We recently characterized a novel roseophage, vB_DshS-R4C (R4C), that could infect the Dinoroseobacter shibae DFL12T, a ubiquitous group of Gram-negative α-proteobacteria of the Roseobacter clade. Here, we report the atomic capsid and in-situ structures of the tail machine of the marine siphophage, vB_DshS-R4C (R4C), which infects Roseobacter. The R4C virion, comprising 12 distinct structural protein components, has a unique five-fold vertex of the icosahedral capsid that allows genome delivery. In this study, we use cryo-electron microscopy (cryo-EM) and structure prediction to determine the atomic structure of the phage R4C capsid and the in-situ structure of the tail machinery to characterize the distinguished long rigid tail.

The C12 reconstruction of the portal-adaptor complex, with an overall resolution of 4.7 Å, characterizes an adaptor architecture that decorates an accessory Ig-like domain at its periphery. The R4C portal protein, forming a canonical cone-shaped dodecamer with a height of 10 nm, shows considerable structural similarity with portal proteins of other phages, despite poor sequence conservation. The portal protein, characterized from top to bottom, comprises separate crown (residues 476–551), wing, stem, and clip domains (324–376)51. A typical tunnel loop connecting α8 forms the narrowest channel with a diameter of ~30 Å; an analogous structural feature (e.g., phages SPP1 and T4) confines the DNA and prevents its reflux from the capsid, with the specific conformational rearrangement in the tunnel loop regulating genome release. The clip domain, straddling the thick capsid wall, is partially exposed outside the R4C head and interacts with the adaptor proteins. The portal complex is capped by a dodecameric adaptor, which is located outside the capsid shell and interacts with both the portal and the capsid MCPs. Following the nomenclature established for the RcGTA adaptor, the R4C adaptor protein can be divided as: attachment domain (1–106), tube domain, adaptor loop (131–148) and C-terminal hook (167–178). The N-terminus of the adaptor protein is an immunoglobulin (Ig)-like domain (attachment domain), and this domain is connected to the tube domain by a long, flexible loop. The tube domain consists of two α-helices, with the α2 sandwiched between loops from adjacent portal proteins. The tube domain extends the C-terminal hook to the portal clip domain, forming an interaction network comprising five hybrid β-sheets.

>[12x]MRFWPFSKTTNAATRAEPMVTRPDTAPRVRSYRAAKSDRIAGGFGVFPTTPRDELRREIRGLVGHSRHAAQNFDYARAYEMLTRRHVIGFNGIRLQMDVRDPGGKKDVAAGAQIESAWARWGKMKNSPTPCGRLSWWGVECQVATGIAREGGSFVRIHQGTNRGRFGFQVEPIPFDLLDLDLTGPTPGGGFVGIAREGGSFVRIHQGTNRGRFGFQVEPIPFDLLDLDLTGPTPGGGFVESGVEFDATDRVVAYHMWSAAMSEGHRPGARRRLRIPAAQMLYVLVPEEIGQALGVPRSATALRLMNLSEKFQESALTAANYGASNMVFFERAADNGVVTGPEDDAQIPIDQIEAGTLTELPPGVKAVSHNPAYPDAAVGPFLRQMGTSQAAGLGVSYETLTADLSGANFSSLRAGKGEEREEWRMLQRAVFEGLHDRVFSRWLPLAMLSGEVRLPLAKLDKFDAATWRPRGWPSVNPKDDATAHEKDLKNGVRTRTEICAERGRDFADVVAEAAAERQMMRDAGLDPDAPLRTSPPETPPDPGEEIEGKDT;>MTVSIHPPATLVAGDSWAWEAGAVFEDHPDPWAASYVLRPEAGGDPVTVSGGLEVLAPVFRLPASVTADLPPGEWTWFAVAVDATTDARAVLAQGRVTVIPDPLAGTEDRRTPARRILAAIEATLEGRATKDADTYSIEGRSITRTPLPDLLRLRAVYAEQVARETGRSPYRQRRVSF[12x]>MAGARQELDTFTRGLKGLDGQFSQRVTDANGRVKENSSGRVALATPRQFRWEYAKPYKQLIVADGKKVWVFDPDLEQVTVRAQGSEEQNSPLVALIDPTRLDKQYDVSEEAAPRDGLQWLSLTPKVDTDASFQMASLGFGKDGLAKMEVVDAVGQRTAISFSGWKRNPAFAADTFRYTPGKGVDVVGDAQAENLYFQSHHHHHH[2x];>MVSVPRGQGGAAPAVVGQVSESARQAEAARQAWLQAHPAWSFQGRVAISKGRDGGSGRLDWQQDGPRYHVQLSAPVTRQSWVLTGDTTTGAGRLEGLDGGPRAGADAEQVLLEATGWTIPVNQMPDWVRALRIADAGAARVDLDEHGRPRTVQQDGWTIDFLEWTPASAAQPELPRRIEARNGDAKVRLLVDQWTLSPAENLYFQSHHHHHH[2x]

The LPs are localized to the OM where they are attached via a lipid anchor by a process known as the localization of lipoprotein (Lol) pathway. The ABC extractor presents the extracted LP to the transport protein LolA, which binds the anchor and thereby shields it from the hydrophilic periplasmic milieu. At the periplasmic face of the OM, the LP cargo is delivered to LolB, which completes the Lol pathway by inserting the LP anchor in the inner leaflet of the outer membrane. As most Gram-negative bacterial pathogens, the genome of the phytopathogen Xcc contains genes coding for a tripartite Lol system with an ABC-type extractor, the LolA chaperone and the OM insertase LolB.

In the present study, we present the experimental crystal structure of the LP-free LolA-LolB complex from Xanthomonas campestris pv. campestris. The crystal structure of the Xcc LolA-LolB complex was determined in the trigonal crystal form R3 with two LolA-LolB heterodimers in the asymmetric unit. LolA-LolB heterodimer 1 (LolA1-LolB1) consists of chains A and B, and LolA-LolB heterodimer 2 (LolA2-LolB2) of chains C and D. In both heterodimers, LolA and LolB interact in a “mouth-to-mouth” orientation with the LolB hook inserted between the two β-sheets of LolA, similar to what was first proposed by Okuda and Tokuda. A six-residue long loop between β3B and β4B in LolB (residues 74–79) forms a hook that inserts like a wedge between the two β-sheets in LolA. An annular opening is formed on one face of the LolA-LolB complex. In the lipid-free LolA-LolB complex, both paths that lead from the annulus to the hydrophobic cavities in LolA and LolB are closed off. The path leading to the LolA cavity is blocked by residues in the LolA lid domain and the LolB hook, and the path to the LolB cavity is blocked by Trp81 in LolB. The LolB hook (residues 74–79 in chains B and D) assumes slightly different conformations in the two heterodimers to allow some conformational freedom when docked to LolA in the absence of bound lipid. Due to the different conformation of the LolB hook in the two non-crystallographically related heterodimers, LolA and LolB in heterodimer 1 (chains A and B) are slightly more tightly associated than LolA and LolB in heterodimer 2 (chains C and D).The eukaryotic translation initiation factor 4E (eIF4E) protein is a vital component of the cap-dependent mechanism for mRNA translation. It binds the 7-methylguanosine (m7G) cap structure present at the 5′ end of mRNA molecules and recruits it as part of the eIF4F assembly which also includes two other partner proteins, eIF4A and eIF4G, to the translational machinery for protein synthesis. We have used a structure-guided approach to rationally develop a set of hydrocarbon stapled-peptides with high binding affinities and residence times against the oncogenic eukaryotic translation initiation factor 4E (eIF4E) protein. Crystal structures of these peptides in complex with eIF4E show that they form specific interactions with a region on the protein-binding interface of eIF4E which is distinct from the other well-established canonical interactions.

Two 15mer peptide derivatives of sTIP-05 (sTIP-09: 1KKRYSR*QLL*FRRR15 and sTIP-10: 1KKRYSREQLL*FQR*15) were synthesized, one with an “13RRR15” sequence extension and the other with an i, i + 4 hydrocarbon staple shifted to positions 11 and 15 of the peptide sequence which encapsulates the “12FQR14” sequence at the C-terminus. In sTIP-10, position 7 was substituted by a glutamic acid (E7) as is seen in the sequence of the parent eIF4G1 peptide. Significantly though, their rates of dissociation decreased relative to sTIP-05 and hence residence times were improved (68 seconds for sTIP-09 and 39 seconds for sTIP-10). The crystal structure of sTIP-10 with eIF4E showed that the helical content of this peptide was relatively higher than in the other peptides because the i, i + 4 hydrocarbon staple stabilized an additional helical turn in the extended C-terminus of the peptide. However, this staple linker was still exposed to the solvent as observed in the other crystal structures, with no interactions made with the protein. The side-chain of Q13 behaved similar to W13 in sTIP-07 and R13 in sTIP-09, forming hydrogen-bond interactions with N77 and hydrophobic interactions with residues W73, Y76 and L131. Residue R14, being exposed to the solvent, did not form any specific interactions with eIF4E but should contribute to peptide solubility. MD simulations of the sTIP-10 and eIF4E crystal structure showed that the peptide maintained the additional helical turn observed at the C-terminus primarily because of the stability provided by the hydrocarbon linker (Movie S6†). Residue Q13 in the extended terminal segment contributed favorably (–2.0 kcal mol–1) to binding through its predominantly hydrophobic interactions with eIF4E along with the core residues (Y4, R6, L9, L10 and F12; –2.1 to –6.9 kcal mol–1) in the peptide.

> MVANPEHYIKHPLQNRWALWFFKNDKSKTWQANLRLISKFDTVEDFWALYNHIQLSSNLMPGCDYSLFKDGIEPMWEDEKNKRGGRWLITLNKQQRRSDLDRFWLETLLCLIGESFDDYSDDVCGAVVNVRAKGDKIAIWTTECENREAVTHIGRVYKERLGLPPKIVIGYQSHADTATKSGSTTKNRFVV;> XKKRYSREQLLLFQRLX>MKSMSEYLNLLKEAIQNVVDGGWHETKRKGNTGIGKTFEDLLEKEEDNLDAPDFHDIEIKTHETAAKSLLTLFTKSPTNPRGANTMLRNRYGKKDEYGNNILHQTVSGNRKTNSNSYNYDFKIDIDWESQVVRLEVFDKQDIMIDNSVYWSFDSLQNQLDKKLKYIAVISAESKIENEKKYYKYNSANLFTDLTVQSLCRGIENGDIKVDIRIGAYHSGKKKGKTH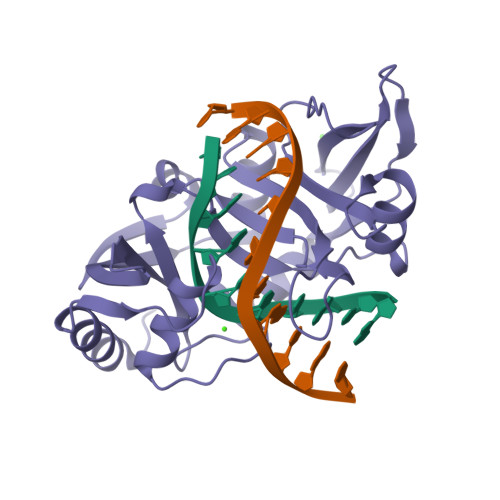DHGTAFRINMEKLLEYGEVKVIV[2x]>SAAATQAVPAPNQQPEVFCNQIFINNEWHDAVSRKTFPTVNPSTGEVICQVAEGDKEDVDKAVKAARAAFQLGSPWRRMDASHRGRLLNRLADLIERDRTYLAALETLDNGKPYVISYLVDLDMVLKCLRYYAGWADKYHGKTIPIDGDFFSYTRHEPVGVCGQIIPWNFPLLMQAWKLGPALATGNVVVMKVAEQTPLTALYVANLIKEAGFPPGVVNIVPGFGPTAGAAIASHEDVDKVAFTGSTEIGRVIQVAAGSSNLKRVTLELGGKSPNIIMSDADMDWAVEQAHFALFFNQGQCCCAGSRTFVQEDIYDEFVERSVARAKSRVVGNPFDSKTEQGPQVDETQFKKILGYINTGKQEGAKLLCGGGIAADRGYFIQPT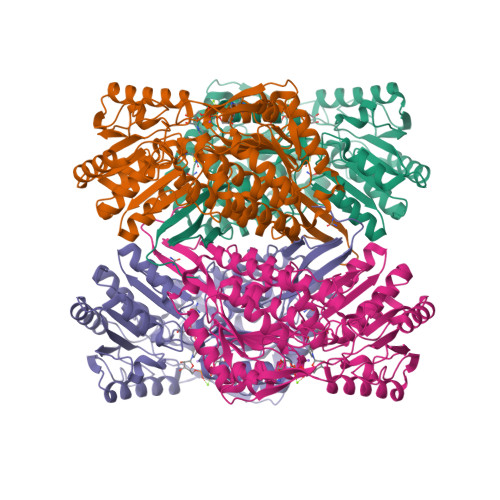VFGDVQDGMTIAKEEIFGPVMQILKFKTIEEVVGRANNSTYGLAAAVFTKDLDKANYLSQALQAGTVWVNCYDVFGAQSPFGGYKMSGSGRELGEYGLQAYTEVKTVTVKVPQKNS[4x]>ADFEVHMLNKGKDGAMVFEPASLKVAPGDTVTFIPKDKGHNVETIKGMIPDGAEAFKSKINENYKVTFTAPGVY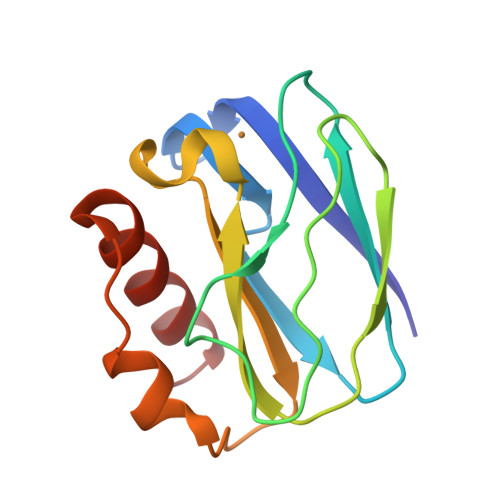GVKCTPHYGMGMVGVVQVGDAPANLEAVKGAKNPKKAQERLDAALAALGN[4x]(2~{S})-~{N}-(4-ethanoyl-1,3-thiazol-2-yl)piperazine-2-carboxamide | C10 H14 N4 O2 S | 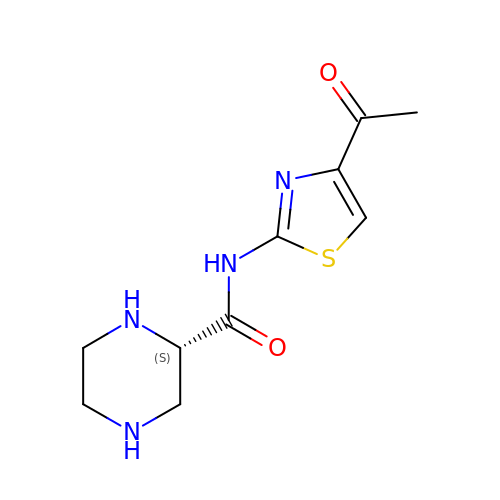AESXBAWWRWZMPF-ZETCQYMHSA-N>[2x]MGDEDKRITYEDSEPSTGMNYTPSMHQEAQEETVMKLKGIDANEPTEGSILLKS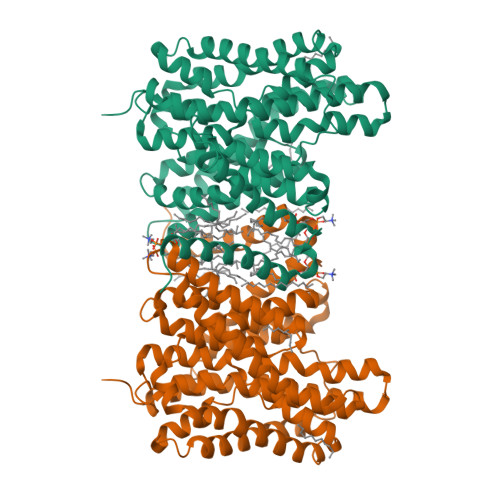SEKKLQETPTEANHVQRLRQMLACPPHGLLDRVITNVTIIVLLWAVVWSITGSECLPGGNLFGIIILFYCAIIGGKLLGLIKLPTLPPLPSLLGMLLAGFLIRNIPVINDNVQIKHKWSSSLRSIALSIILVRAGLGLDSKALKKLKGVCVRLSMGPCIVEACTSALLAHYLLGLPWQWGFILGFVLGAVSPAVVVPSMLLLQGGGYGVEKGVPTLLMAAGSFDDILAITGFNTCLGIAFSTGSTVFNVLRGVLEVVIGVATGSVLGFFIQYFPSRDQDKLVCKRTFLVLGLSVLAVFSSVHFGFPGSGGLCTLVMAFLAGMGWTSEKAEVEKIIAVAWDIFQPLLFGLIGAEVSIASLRPETVGLCVATVGIAVLIRILTTFLMVCFAGFNLKEKIFISFAWLPKATVQAAIGSVALDTARSHGEKQLEDYGMDVLTVAFLSILITAPIGSLLIGLLGPRLLQKVEHQNKDEEVQGETSVQV>GHMAPAPPANSGESSLLSESELPAGISYAEAMEGGSRPLLHPDNPVVFFDISIGSHEAGRIKIELFKNLAPKSAENFRQFCTGEFRQNQVPIGYKGATFHRIIKNFMIQGGDFVKGDGTGRLSIYGSSFPDEAFVLPHFRSGLLSLANSGPDTNGCQFFITCAKCDWLNRKHVVFGQV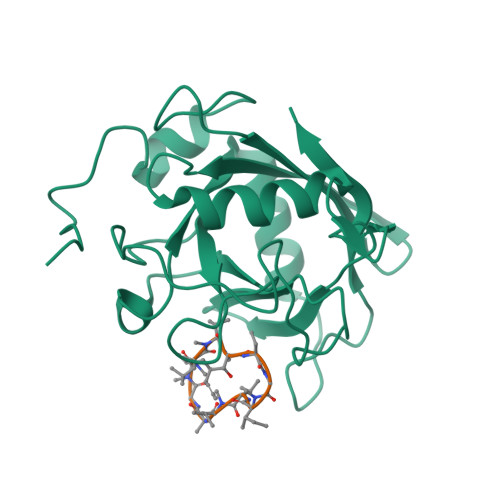LGKESMQVVRKIEHVTVDGGNRPRIPVTVTQCGEL[2x];>[2x]ALLVTAGIVLA> MKKQNDIPQPIRGDKGATVKIPRNIERDRQNPDMLVPPETDHGTVSNMKFSFSDTHNRLEKGGYAREVTVRELPISENLASVNMRLKPGAIRELHFHKEAEWAYMIYGSARVTIVDEKGRSFIDDVGEGDLWYFPSGLPHSIQALEEGAEFLLVFDDGSFSENSTFQLTDWLAHTPKEVIAANFGVT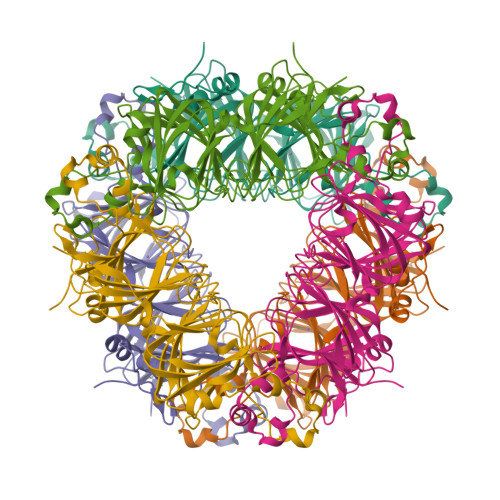KEEISNLPGKEKYIFENQLPGSLKDDIVEGPNGEVPYPFTYRLLEQEPIESEGGKVYIADSTNFKVSKTIASALVTVEPGAMRELHWHPNTHEWQYYISGKARMTVFASDGHARTFNYQAGDVGYVPFAMGHYVENIGDEPLVFLEIFKDDHYADVSLNQWLAMLPETFVQAHLDLGKDFTDVLSKEKHPVVKKKCSK>MSALFEPYTLKDVTLRNRIAIPPMCQYMAEDGLINDWHQVHYASMARGGAGLLVVEATAVAPEGRITPGCAGIWSDAHAQAFVPVVQAIKAAGSVPGIQIAHAGRKASANRPWEGDDHIGADDARGWETIAPSAIAFGAHLPNVPRAMTLDDIARVKQDFVDAARRARDAGFEWIELHFAHGFLGQSFFSEHSNKRTDAYGGSFDNRSRFLLETLAAVREVWPENLPLTARFGVLEYDGRDEQTLEESIELARRFKAGGLDLLSVSV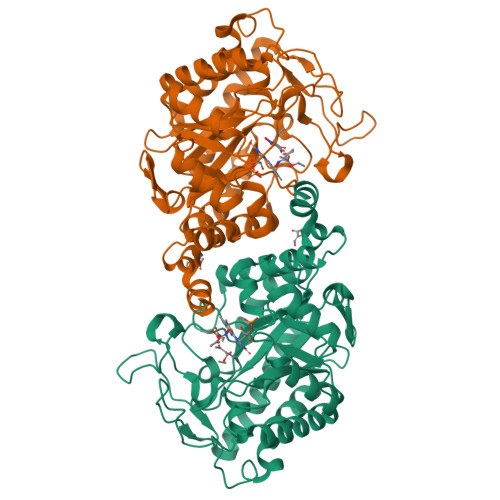GFTIPETNIPWGPAFMGPIAERVRREAKLPVTSAWGFGTPQLAEAALQANQLDLVSVGRAHLADPHWAYFAAKELGVEKASWTLPAPYAHWLERYRLEHHHHHH[2x]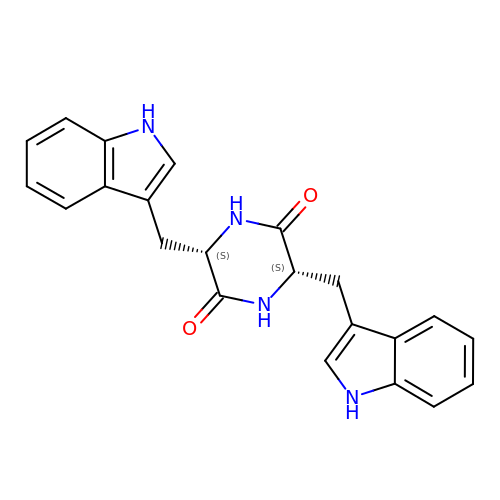(3S,6S)-3,6-bis[(1H-indol-3-yl)methyl]piperazine-2,5-dione | C22 H20 N4 O2 | DNHODRZUCGXYKU-PMACEKPBSA-N>[2x]SQIRHYKWEVEYMFWAPNCNENIVMGINGQFPGPTIRANAGDSVVVELTNKLHTEGVVIHWHGILQRGTPWADGTASISQCAINPGETFFYNFTVDNPGTFFYHGHLGMQRSAGLYGSLIVDPPQGKKEPFHYDGEINLLLSDWWHQSIHKQEVGLSSKPIRWIGEPQTILLNGRGQFDCSIAAKYDSNLEPCKLKGSESCAPYIFHVSPKKTYRIRIASTTALAALNFAIGNHQLLVVEADGNYVQPFYTSDIDIYSGESYSVLITTDQNPSENYWVSVGTRARHPNTPPGLTLLNYLPNSVSKLPTSPPPQTPAWDDFDRSKNFTYRITAAMGSPKPPVKFNRRIFLLNTQNVINGYVKWAINDVSLALPPTPYLGAMKYNLLHAFDQNPPPEVFPEDYDID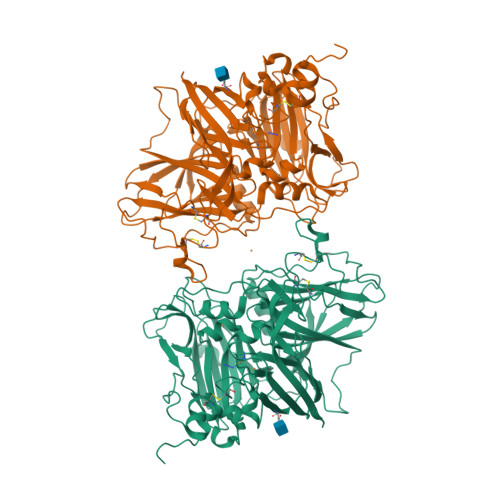TPPTNEKTRIGNGVYQFKIGEVVDVILQNANMMKENLSETHPWHLHGHDFWVLGYGDGKFSAEEESSLNLKNPPLRNTVVIFPYGWTAIRFVADNPGVWAFHCHIEPHLHMGMGVVFAEGVEKVGRIPTKALACGGTAKSLINNPKNP>CCTAATTA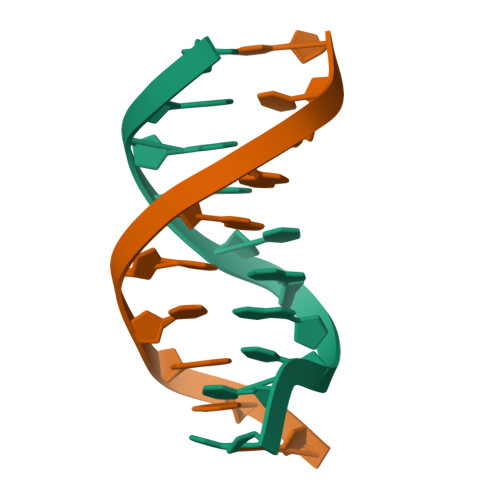GG[2x]The Mad1‐Mad2 complex, which is required to catalyse MCC formation, is targeted to kinetochores through a direct interaction with the phosphorylated conserved domain 1 (CD1) of Bub1. Mad1CTD is comprised of an N‐terminal elongated coiled‐coil, followed by a globular head domain featuring a conserved RWD (RING, WD40, DEAD) domain. Each monomer contains a long N‐terminal α‐helix (α1) forming the stem, followed by an antiparallel β‐sheet of four β‐strands (β1–4), a short helix (α2) and two C‐terminal helices (α3/α4). Bub1CD1 is largely a single α‐helix, consisting of almost four turns.

The highest resolution crystal structure, belonging to space group P212121, diffracted to 1.75 Å, with one Mad1CTD‐Bub1CD1 complex per asymmetric unit. In the crystal structure, two Bub1CD1 peptides are bound to the Mad1CTD homodimer. Unexpectedly, the peptide binding interface lies diagonally across the Mad1CTD coiled‐coil, making contacts with both Mad1CTD monomers. The start of the CD1 helix begins with the phosphothreonine residue (pThr461), contacting the coiled‐coil of one monomer at the conserved Mad1 RLK motif, whereas its C‐terminus contacts the opposite Mad1 subunit at the top of the coiled‐coil and its adjoining head domain β‐sheet. Specifically, the phosphate group of pThr461 forms a direct interaction with Mad1 through a charged hydrogen bond with Arg617 of the conserved Mad1 RLK motif. Our structure further reveals that pSer459 does not contact Mad1; instead, it is part of the disordered N‐terminal tail of Bub1CD1. A striking feature of the pThr461 residue is its position at the start of the CD1 helix. Here, the phosphate group caps the N‐terminus of the helix, stabilizing the positively charged helix dipole with its bulky negative charge. In our crystal structure, where Bub1CD1 and Mad1CTD are co‐crystallized at concentrations over 100 times the KD and with a sevenfold molar excess of peptide, we see clear differential occupancy of the peptides in the electron density map and the 2Fo‐Fc omit map (Figs EV2A and C, and D). Significantly, the side of the coiled‐coil which angles inwards comprises the binding site of the higher occupancy peptide, whereas the lower, partial occupancy peptide binds to the outside of the bend.

>SSKEVAELKKQVESAELKNQRLKEVFQTKIQEFRKACYTLTGYQIDITTENQYRLTSLYAEHPGDCLIFKATSPSGSKMQLLETEFSHTVGELIEVHLRRQDSIPAFLSSLTLELFSRQTVA[2x];>[2x]KVQPSPTVHTKEALGFIMNMFQAPTS Staphylococcus epidermidis expresses glycerol phosphate wall teichoic acid (WTA), but some health care–associated methicillin-resistant S. epidermidis (HA-MRSE) clones produce a second, ribitol phosphate (RboP) WTA, resembling that of the aggressive pathogen Staphylococcus aureus. We report here that the TarM enzyme of HA-MRSE [TarM(Se)] glycosylates RboP-WTA with glucose, instead of N-acetylglucosamine (GlcNAc) by TarM(Sa) in S. aureus. Each blade of the homotrimer contains a catalytic domain with a canonical GT-B fold, consisting of an N-terminal acceptor substrate-binding domain (ABD; residues 1 to 68 and 202 to 302) and a C-terminal nucleotide-binding domain (residues 303 to 492). TarM(Se) is a retaining WTA glycosyltransferase; therefore, the relative positions of donor and acceptor substrates in TarM(Se) and TarP are different.

The backbone amide and carbonyl groups of Thr383 form two hydrogen bonds with the O2 and N3 atoms of the base, providing specificity for uridine, and the aromatic ring system of the base is stacked against the Tyr382 side chain. The tandem backbone amide groups of Leu407 and Ser408 contact the α-phosphate of UDP-glucose and another main-chain amide group from Gly17 interacts with β-phosphate. In addition, the side chains of Arg326 and Lys331, each form two salt bridges with the β-phosphate. The glucose moiety contacts TarM(Se)G117R through multiple interactions. The side chains of Asn304 and His249 are hydrogen-bonded to the C6 hydroxyl group, the backbone amide group of Gly406 interacts with C4 hydroxyl, and the Glu403 side chain and backbone amide groups of Gly404 and Gln405 contact with the C3 hydroxyl group. The side chain of Gln330 is hydrogen-bonded to the C2 hydroxyl. The related enzyme TarM(Sa), which accepts UDP-GlcNAc as donor substrate, has a threonine at this position. Thus, the longer Gln330 side chain appears to allow TarM(Se) to distinguish UDP-glucose from UDP-activated bulkier sugars, such as UDP-GalNAc and UDP-GlcNAc. The binding site for UDP-glucose in TarM(Se) is composed of eight amino acids, seven of which are identical to that for UDP-GlcNAc in TarM(Sa). The only difference is Gln330 in TarM(Se) and Thr330 in TarM(Sa), which clearly suggests a key role for this residue in allowing TarM(Se) to discriminate against the use of UDP-GlcNAc as a donor substrate.

> MHHHHHHSGENLYFQSMKQTYMIVNELDVNKGGMTTAMLTRSKFFLDNEISGDIITFDFKANYKDILKELVQSKKMDKRTQMHNPFIYFKNISNLQHKKYNYTMTRNLSNLLKDSVEIKENSRISRFFNIMSREYLAYKRETEQETIFDLFKNNLRYKRIYFYKGKIVKTEVFNSDNNLIAEQFYDDNGYLYLYRQINPEKKSIGKTYLVCKEKQFKNNVEFCSYFLDKLIPDINDNIIICDGPGSFPKILKTNHKNVKKFAVIHVNHYKNFDDTGAVKKQEDYILRNANKINGVVMLTEAQKKDIIEKYKITNAYVISNFINITDDYRDKNDNKVVGHISRLVPQKGLPYLIDVAKKVVEQDNSVEFHLYGTGEEKSKIENLIQESNLTNNVKLLGYTTNAIEKIKDFRCVISTSQFEGQGLSLIEAMLLKKPVVAFDVKYGPSDFVKDGKNGYLIENKDIKKMANKILKLLHDKELSKSLGKHGRDTIIDMYQPEKLMVKWKQLFN> VASYDYLVIGGGSGGLASARRAAELGARAAVVESHKLGGTCVNVGCVPKKVMWNTAVHSEFMHDHADYGFPSCEGKFNWRVIKEKRDAYVSRLNAIYQNNLTKSHIEIIRGHAAFTSDPKPTIEVSGKKYTAPHILIATGGMPSTPHESQIPGASLGITSDGFFQLEELPGRSVIVGAGYIAVEMAG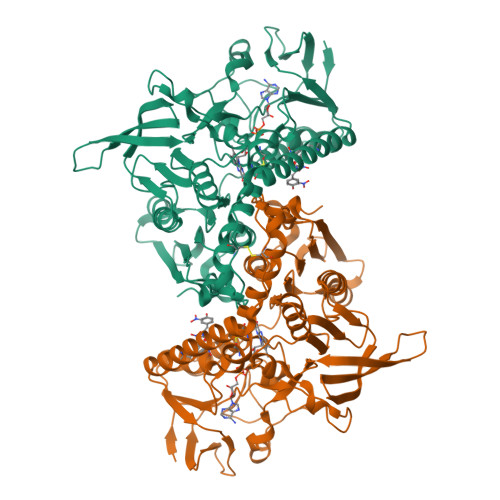ILSALGSKTSLMIRHDKVLRSFDSMISTNCTEELENAGVEVLKFSQVKEVKKTLSGLEVSMVTAVPGRLPVMTMIPDVDCLLWAIGRVPNTKDLSLNKLGIQTDDKGHIIVDEFQNTNVKGIYAVGDVCGKALLTPVAIAAGRKLAHRLFEYKEDSKLDYNNIPTVVFSHPPIGTVGLTEDEAIHKYGIENVKTYSTSFTPMYHAVTKRKTKCVMKMVCANKEEKVVGIHMQGLGCDEMLQGFAVAVKMGATKADFDNTVAIHPTSSEELVTLR> MFAFYFLTACISLKGVFGVSPSYNGLGLTPQMGWDNWNTFACDVSEQLLLDTADRISDLGLKDMGYKYIILDDCWSSGRDSDGFLVADEQKFPNGMGHVADHLHNNSFLFGMYSSAGEYTCAGYPGSLGREEEDAQFFANNRVDYLKYDNCYNKGQFGTPEISYHRYKAMSDALNKTGRPVFYSLCNWGQDLTFYWGSGIANSWRMSGDVTAEFTRPDSRCPCDGDEYDCKYAGFHCSIMNILNKAAPMGQNAGVGGWNDLDNLEVGVGNLTDDEEKAHFSMWAMVKSPLIIGANVNNLKASSYSIYSQASVIAINQ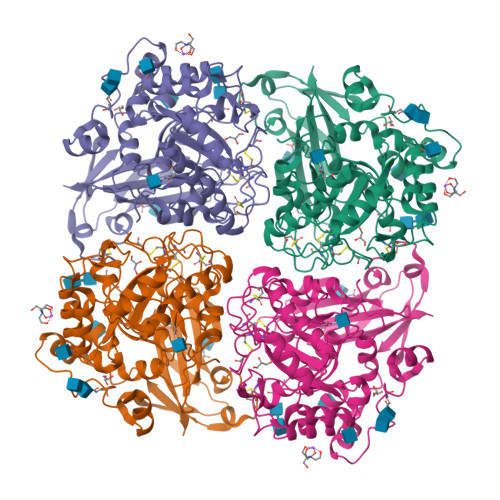DSNGIPATRVWRYYVSDTDEYGQGEIQMWSGPLDNGDQVVALLNGGSVSRPMNTTLEEIFFDSNLGSKKLTSTWDIYDLWANRVDNSTASAILGRNKTATGILYNATEQSYKDGLSKNDTRLFGQKIGSLSPNAILNTTVPAHGIAFYRLRPSSDYKDDDDK> ETVPVKLKPGMDGPKVKQWPLTEEKIKALVEICTEMEKEGKISKIGPENPYNTPVFAIKKKDSTKWRKLVDFRELNKRTQDFWEVQLGIPHPAGLKKKKSVTVLDVGDAYFSVPLDEDFRKYTAFTIPSINNETPGIRYQYNVLPQGWKGSPAIFQSSMTKILEPFRKQNPDIVIYQYMDDLCVGSDLEIGQHRTKIEELRQHLLRWGLTTPDKKHQKEPPFLWMGYELHPDKWTVQPIVLPEKDSWTVNDIQKLVGKLNWASQIYPGIKVRQLCKLLRGTKALTEVIPLTEEAELELAENREILKEPVHGVYYDPSKDLIAEIQKQGQGQWTYQIYQEPFKNLKTGKYARMRGAHTNDVKQLTEAVQKI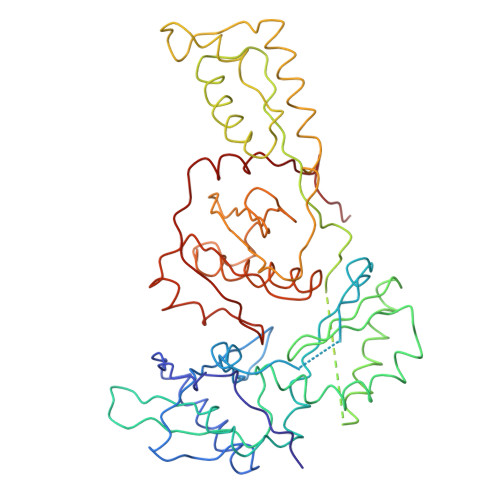TTESIVIWGKTPKFKLPIQKETWETWWTEYWQATWIPEWEFVNTPPLVKLWYQLEKEPIVGAETF> ANIVGGIEYSINNASLCSVGFSVTRGATKGFVTAGHCGTVNATARIGGAVVGTFAARVFPGNDRAWVSLTSAQTLLPRVANGSSFVTVRGSTEAAVGAAVCRSGRTTGYQCGTITAKNVTANYAEGAVRGLTQGNACAGRGDSGGSWITSAGQAQGVMS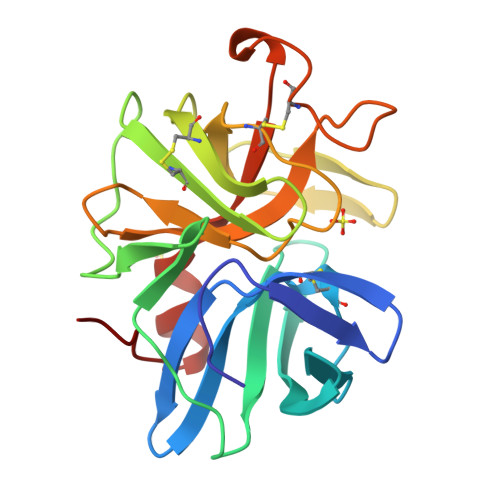GGNVQSNGNNCGIPASQRSSLFERLQPILSQYGLSLVTG>[2x]MVHYKLTYFNGRGAAEIIRQVFVLAGQDYEDVRLTHEEWPKHKASMPFGQLPV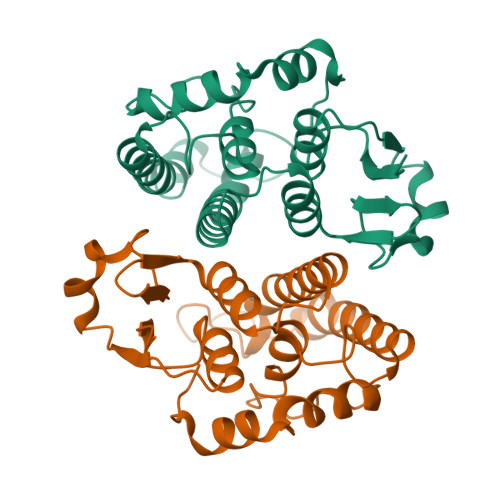LEVDGKQLPQSVAIVRYLARKFGYAGKSAWEEAVVDSIADQFKDFLNEVRPYFKVLLGMDQGDLKALEKDVFEPARQKFFTIVTKILKENKTGYLVGDSLTFADLYVAEMGFTEHYPKLYDGFPEVKAHAEKVRSNPKLKKWIETRPASKF2-chloro-4-{[(3S)-1-methylpyrrolidin-3-yl][2-(trifluoromethyl)benzyl]amino}benzonitrile 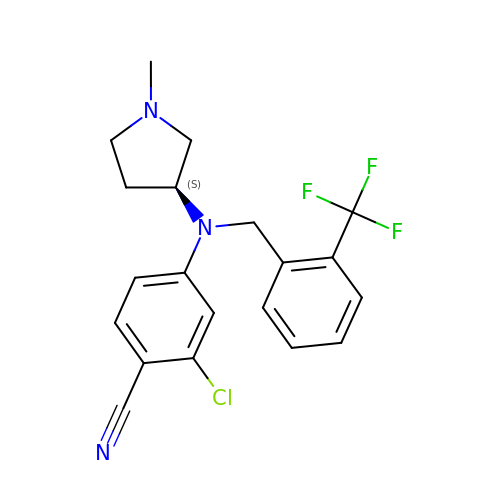| C20 H19 Cl F3 N3 | HMOAZJHSXXENHE-KRWDZBQOSA-N>[4x]MSQHNEKNPHQHQSPLHDSSEAKPGMDSLAPEDGSHRPAAEPTPPGAQPTAPGSLKAPDTRNEKLNSLEDVRKGSENYALTTNQGVRIADDQNSLRAGDRGPTLLEDFILREKITHFDHERIPERIVHARGSAAHGYFQPYKSLSDITKADFLSDPNKITPVFVRFSTVQGGAGSADTVRDIRGFATKFYTEEGIFDLVGNNTPIFFIQDAHKFPDFVHAVKPEPHWAIPQGQSAHDTFWDYVSLQPETLHNVMWAMSDRGIPRSYRTMEGFGIHTFRLINASGKATFVRFHWK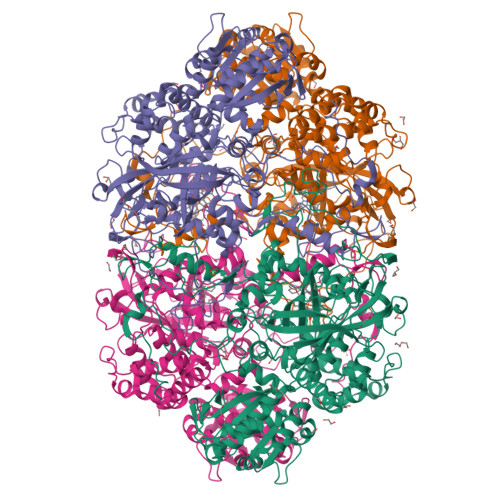PLAGKASLVWDEAQKLTGRDPDFHRRELWEAIEAGDFPEYELGFQLIPEEDEFKFDFDLLDPTKLIPEELVPVQRVGNMVLNRNPDNFFAENEQAAFHPGHIVPGLDFTNDPLLQGRLFSYTDTQISRLGGPNFHEIPINRPTCPYHNFQRDGMHRMGIDTNPANYEPNSINDNWPRETPPGPKRGGFESYQERVEGNKVRERSPSFGEYYSHPRLFWLSQTPFEQRHIVDGFSFELSKVVRPYIRERVVDQLAHIDLTLAQAVAKNLGISLTDDQLNITPPPDVNGLKKDPSLSLYAIPDGDVKGRVVAILLNDEVRSADLLAILKALKAKGVHAKLLYSRMGEVTADDGTVLPIAATFAGAPSLTVDAVIVPCGNIADIADNGDANYYLMEAYKHLKPIALAGDARKFKATIKVADQGEEGIVEADSADGSFMDELLTLMAAHRVWSRIPKIDSIPA>[3x]RARHKISRAGVELIKSFEGLRQQASQLPDGRWMIGYGHTFSAREGARVTAEDADALLRFDL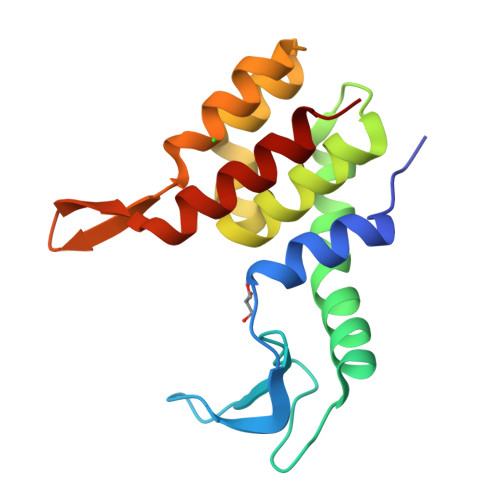LPIVEAVNNLVHTPLTQNQFDALVSFCFNIGIEAFGQSDVLRRVNEGRVTEAAQAMDNWTSAEFNGQTYVLAPLIRRRASEKSLFLTP>MPLLVEGRRVRLPQSAGDLVRAHPPLEERARLLRGQSVQQVGPQGLLYVQQRELAVTSPKDGSISILGSDDATTSHIVVLRHTGNGATCLTHCDGTDTKAEVPLIMNSIKSFSDHAQCGRLEVHLVGGFSDDRQLSQKLTHQLLSEFDRQEDDIHLVTLCVTELNDREENENHFPVIYGIAVNIKTAEIYRASFQDRGPEEQLRAARTLAGGPMISIYDAETEQLRIGPYSWTPFPHVDFWLHQDDKQILENLSTSPLAEPPHFVEHIRSTLMFLKKHPSPAHTLFSGNKALLYKKNEDGLWEKISSPGSLEHHHHHH[2x];>NLAAR[2x]

Especially, exposure or modification of N-terminal amino acid residues can mediate protein degradation and the resultant proteolytic procedure is called the N-degron pathway (formerly the N-end rule pathway). Two tertiary degrons, Asn and Gln, are hydrolyzed into the secondary degron Asp and Glu by N-terminal asparagine amidohydrolase 1 (NTAN1) and N-terminal glutamine amidohydrolase 1 (NTAQ1), respectively. In multicellular eukaryotes, Nt-Asn and Nt-Gln are deamidated by NTAN1-encoded NtN-amidase and NTAQ1-encoded NtQ-amidase, respectively. In this study, the crystal structure of NTAN1, the last veiled structure among three amidases in the N-degron pathway, was elucidated.

Although yNta1, NTAQ1, and NTAN1 do appear to share catalytic functions commonly involving a conserved Cys residue critical for the deamidation activity, they exhibit low sequence similarity to each other. And we explain unexpected substrate specificities of NTAN1 based on structural and biochemical analyses.2,3-dihydroxypropyl (9Z)-octadec-9-enoate | C21 H40 O4 | 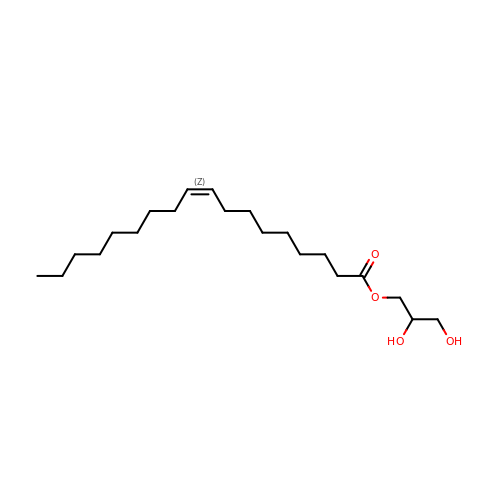RZRNAYUHWVFMIP-KTKRTIGZSA-N> MGHHHHHHSIETDRVSKEFIEFLKTFHKTGQEIYKQTKLFLEGMHYKRDLSIEEQSECAQDFYHNVAERMQTRGKVPPERVEKIMDQIEKYIMTRLYKYVFCPETTDDEKKDLAIQKRIRALRWVTPQMLCVPVNEDIPEVSDMVVKAITDIIEMDSKRVPRDKLACITKCSKHIFNAIKITKNEPASADDFLPTLIYIVLKGNPPRLQSNIQYITRFCNPSRLMTGEDGYYFTNLCCAVAFIEKLDAQSLNLSQEDFDRYMSQMYKNLDLLSQLNERQERIMNEAKKLEKDLIDWTDGIAREVQD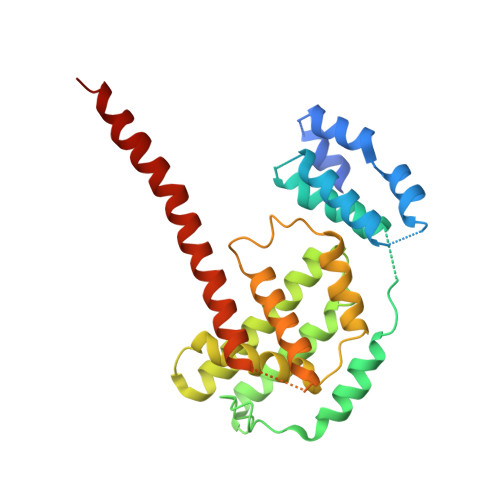IVEK Elongation factor G (EF-G) is a highly conserved and essential GTPase protein that catalyzes tRNA translocation on ribosomes at several stages of protein synthesis. In addition, EF-G is involved in ribosome recycling and suppression of ribosomal frameshifting. Mtb EF-G1 has five structural domains that fold into an elongated shape with dimensions of 118 Å × 60 Å × 50 Å. The N-terminal G domains are composed of a classic GTPase domain (G domain) and an additional G′ subdomain.

We further present the first crystal structure of Mtb EF-G1 in complex with GDP. The crystals of Mtb EF-G1 diffracted the X-ray to 3 Å. However, further crystallographic analysis confirmed that the ASU contained two enzyme molecules with a correct electron density map and reasonable Rwork (20.6%)/Rfree (24.1%) values, instead of a crystallographic monomer in the ASU as in other EF-G structures. The GDP molecule is bound in the G domain. The Walker A motif (23DAGKTT28) forms the A-loop (P-loop), which mainly binds the α- and β-phosphates through main chain atoms in the same way as it does in other EF-G proteins. The O3B, O2B, and O1B atoms of the β-phosphate are specifically recognized by the backbone NH groups of T27, K26, and D23 through multiple hydrogen bonds. The guanosine base is surrounded by several hydrogen bonds donated by S265, F267, and D141. Two interesting parts (switch I and switch II) of the Mtb EF-G1 G domain in molecule A are missing as a result of structural disorder. However, we could model switch II of Mtb EF-G1 in molecule B following refinement. The switch I region of Mtb EF-G1, essential for coupling GTP hydrolysis, was found to be disordered, which is consistent with previous study indicating that the switch I region of EF-G1 has not been modeled, except those in the EF-G in GTP form bound to a ratcheted ribosome and in the S.aureus EF-G structure.

>[2x]MAQKDVLTDLSRVRNFGIMAHIDAGKTTTTERILYYTGINYKIGEVHDGAATMDWMEQEQERGITITSAATTTFWKDNQLNIIDTPGHVDFTVEVERNLRVLDGAVAVFDGKEGVEPQSEQVWRQADKYDVPRICFVNKMDKIGADFYFSVRTMGERLGANAVPIQLPVGAEADFEGVVDLVEMNAKVWRGETKLGETYDTVEIPADLAEQAEEYRTKLLEVVAESDEHLLEKYLGGEELTVDEIKGAIRKLTIASEIYPVLCGSAFKNKGVQPMLDAVVDYLPSPLDVPPAIGHAPAKEDEEVVRKATTDEPFAALAFKIATHPFFGKLTYIRVYSGTVESGSQVINATKGKKERLGKLFQMHSNKENPVDRASAGHIYAVIGLKDTTTGDTLSDPNQQIVLESMTFPDPVIEVAIEPKTKSDQEKLSLSIQKLAEEDPTFKVHLDSETGQTVIGGMGELHLDILVDRMRREFKVEANVGKPQVAYKETIKRLVQNVEYTHKKQTGGSGQFAKVIINLEPFTGEEGATYEFESKVTGGRIPREYIPSVDAGAQDAMQYGVLAGYPLVNLKVTLLDGAYHEVDSSEMAFKIAGSQVLKKAAALAQPVILEPIMAVEVTTPEDYMGDVIGDLNSRRGQIQAMEERAGARVVRAHVPLSEMFGYVGDLRSKTQGRANYSMVFDSYSEVPANVSKEIIAKATGELEGHHHHHH> TGGVQTVTLIPGDGIGPEISAAVMKIFDAAKAPIQWEERNVTAIQGPGGKWMIPSEAKESMDKNKMGLKGPLKTPIAAGHPSMNLLLRKTFDLYANVRPCVSIEGYKTPYTDVNIVTIRENTEGEYSGIEHVIVDGVVASIKLITEGASKRIAEFAFEYARNNHRSNVTAVHKANIMRMSDGLFLQKCREVAESCKDIKFNEMYLDTVCLNMVQDPSQFDVLVMPNLYGDILSDLCAGLIGGLGVTPSGNIGANGVAIFESVHGTAPDIAGKDMANPTALLLSAVMMLRHMGLFDHAARIEAACFATIKDGKSLTKDLGGNAKCSDFTEEICRRVKDLD;> FSEQTIPPSAKYGGRHTVTMIPGDGIGPELMLHVKSVFRHACVPVDFEEVHVSSNADEEDIRNAIMAIRRNRVALKGNIETNHNLPPSHKSRNNILRTSLDLYANVIHCKSLPGVVTRHKDIDILIVRENTEGEYSSLEHESVAGVVESLKIITKAKSLRIAEYAFKLAQESGRKKVTAVHKANIMKLGDGLFLQCCREVAARYPQITFENMIVDNTTMQLVSRPQQFDVMVMPNLYGNIVNNVCAGLVGGPGLVAGANYGHVYAVFETATRNTGKSIANKNIANPTATLLASCMMLDHLKLHSYATSIRKAVLASMDNENMHTPDIGGQGTTSEAIQDVIRHIRVINGRAVEA

Human NAD-dependent isocitrate dehydrogenase or IDH3 (HsIDH3) catalyzes the decarboxylation of isocitrate into α-ketoglutarate in the tricarboxylic acid cycle. It consists of three types of subunits (α, β, and γ) and exists and functions as the (αβαγ)2 heterooctamer. HsIDH3 is regulated allosterically and/or competitively by numerous metabolites including CIT, ADP, ATP, and NADH. In this work, we report the crystal structures of the αβ and αγ heterodimers and the (αβαγ)2 heterooctamer containing an α-Q139A mutation in the clasp domain, which renders all the heterodimers and the heterooctamer constitutively active in the absence of activators.

Crystals of the apo αMγ belong to space group C2, and the asymmetry unit contains one αMγ heterodimer, which forms an (αMγ)2 heterotetramer with a crystallographic 2-fold axis-related heterodimer. However, in the αMγ structure, the γ large domain exhibits an approximate 8° outward rotation from the α-γ interface compared to that in the αMγCIT structure, resulting in an “open” conformation of the allosteric site. Crystal packing analyses show that in the αMγ structure, the γ large domain is involved in close contacts (<4 Å) with the α large domain of a symmetry-related heterodimer and thus its conformation appears to be constrained by the crystal packing; whereas, in the αMγCIT, αMgγ, and αMgγMg+CIT structures (which all adopt the same space group), the γ large domain is not involved in crystal packing and thus its conformation is not constrained. Nevertheless, we cannot exclude the possibility that the conformational flexibility of the γ large domain may play a role in the proper function and catalytic reaction of the αγ heterodimer and the holoenzyme. In the apo αMγ structure, the β3G-α3G and β5G-β6G loops at the allosteric site are partially disordered, whereas in the αMγCIT structure, the β3G-α3G and β5G-β6G loops are well defined in the electron density map. A detailed structural analysis shows that in the αMγ and αMγCIT structures, the hydrogen-bonding networks at the αγ-αγ interface are different from that in the αMgγ structure but similar to that in the αMgγMg+CIT structure. Specifically, the α-Q139A mutation makes Ala139A1 unable to form hydrogen bonds with His131A1 and Ala139A2, and similarly, Ala139A2 cannot form hydrogen bonds with His131A2 and Ala139A1. As a result, the sidechain of His131A1 points toward the α-γ interface and forms a hydrogen bond with the sidechain of His140G2, and the sidechain of His140G1 forms hydrogen bonds with Glu148G1 and Glu148G2; and similarly, the sidechain of His131A2 and His140G2 makes equivalent hydrogen bonds. The His131A-His140G interactions render the β5-β6 loops to adopt active conformations, which lead the sidechains of Tyr126A and Tyr135G to adopt the active conformations as well. In this study, we found that the αMγ heterodimer is constitutively active regardless of the absence and presence of activators.> MDTIAARALTVMRACATLQEARIVLEANVMEILGIAINRYNGLTLRGVTMRPTSLAQRNEMFFMCLDMMLSAAGINVGPISPDYTQHMATIGVLATPEIPFTTEAANEIARVTGETSTWGPARQPYGFFLETEETFQPGRWFMRAAQAATAVVCGPDMIQVSLNAGARGDVQQIFQGRNDPMMIYLVWRR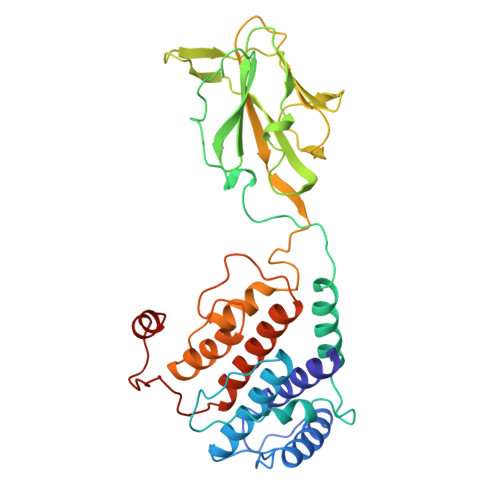IENFAMAQGNSQQTQAGVTVSVGGVDMRAGRIIAWDGQAALHVRNPTQQNAMVQIQVVFYISMDKTLNQYPALTAEIFNVYSFRDHTWHGLRTAIRNRTTLPNMLPPIFPPNDRDSILTLLLLSTLADVYTVLRPEFAMHGVNPMPGPLTAAIARAAYV> GGGCCUAUAGCUCAGGCGGUUAGAGCGCUUCGCUGAUAACGAAGAGGUCGGAGGUUCGAGUCCUCCUAGGCCCACCA;> GGCGACGAUCCGGCCAUCACCGGGGAGCCUUCGGAAGAACGGCGCCGCCGGAAACG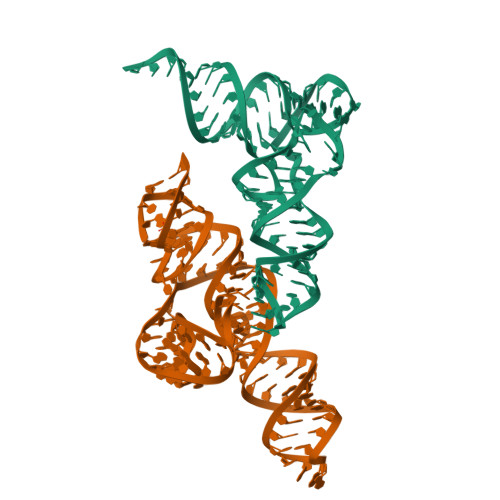GCGGCGCUCAGUAGAACCGAACGGGUGAGCCCGUCACAGCUC Helper NLRs function as central nodes in plant immune networks. Upon activation, they oligomerize into inflammasome-like resistosomes to initiate immune signaling, yet the dynamics of resistosome assembly remain poorly understood. Here, we show that the virulence effector AVRcap1b from the Irish potato famine pathogen *Phytophthora infestans* suppresses immune activation by directly engaging oligomerization intermediates of the tomato helper NLR SlNRC3. Cryo-EM structures of SlNRC3 in AVRcap1b-bound and unbound states reveal that AVRcap1b bridges multiple protomers, stabilizing a stalled intermediate and preventing formation of a functional resistosome.

We purified SlNRC3 activated by PVX-CP and sensor Rx in the presence and absence of AVRcap1b following transient expression in *N. benthamiana* and used cryo-EM to determine the structure of both complexes to understand how the effector could be interfering with immune activation. As in previous work, we used mutants in the MADA motif of the N-terminal α1 helices—which assemble into a funnel-like membrane pore in the resistosome—because they abolish cell death induction without compromising receptor activation or oligomerization. Upon effector or PAMP recognition by intracellular sensors or cell- surface receptors, respectively, resting-state NRC3 dissociates into monomers and assembles into resistosomes in a stepwise manner. The fully assembled complex inserts into the plasma membrane to trigger localized cell death and limit pathogen spread. Previous studies have established that paired NLRs like NLRC4 and NRG1 oligomerize through interactions with heterodimeric (NLRC4-NAIP2) or heterotrimeric (NRG1-EDS1-SAG101) complexes. In contrast, oligomerization of NRC helpers doesn’t involve additional partner proteins. The helper NLRs dissociate to assemble the resistosome independently, with no evidence of sensor-mediated nucleation.

>[6x]MADVAVKFELENETQLEIDNADLILGIQGEVENLLTDLNYFNAFLKEAAKSRRENEVLKELVKKIRKVVNDAEDSIDKFVVEAKRHDDKNKFAQWFHITHVARAKGVADEIKSIRERVKEIRDNDAYGLQAITLDDNFNRGDEERKAPVVEEDDVVGFDDEAKTVIDRLIGGSDYVEVVPVVGMPGLGKTTLAYKIYKDPKVEYEFFTRVWVYVSQTFKRREIFLNIISKFTRNTKQYDDTPEDDLANEVKELLGKGGKYLIVLDDVWTMEAWDRIKIAFPNNGKRNRVLMTTRQSNVAKRCNDKPHDLKFLTKDESWELLEKKVFHKEKCPPELELPGISIAEKCMGLPLAIVVIAGALIGKGKTTREWELVAASVGEHLINRDPENCKKLVQMSYDRLPYDLKACFLYCGAFPGGSQIPAKKLIRLWIAEGFIQYQGPLALEDVAEDHLNDLVNRNLVMVTQRSCSGQIKTCRVHDMLHEFCRHEAMMEENLFQEIKQGQERSFPGKQELATYRRLCIQSLIPEFLSMKPSGEHVRSFLCVGSKKIDMPPNEIPSIPKAFPLLRVLDAESIKFSRFSREFFKLFHLRYIALSTDKIKTIPADFGNLWNIQTLIVETQQATLDIKADIWNMTRLRHVCTNASATLPSTKRPKSSKDNLVNRCLQTLSTIAPECCTAEVFTRTPNLKKLGVRGKIDALLESSKDGSGSGLFSNIGKLGCLEYLKLVNDTRLSSKPLHLPPAYIFPQKLKKLSLVDTWFEWKDMSILGLLPELEVLKLKENAFKGQSWEQEDGGFPRLQVLWIERTDLTSWKASSGNFPRLKHLALISCDKLEELPAELADVKNLQLIELQSSSESAARSARAILKRNQEKEQDGDKGTGFKLSIFPHDLGLSDYKDHDGDYKDHDLDAAAADYKDDDDK>MEQRETIMLPGSDYNHWLIVMEFPKDPAPSRDQMIDTYLNTLATVLGSMEEAKKNMYAFSTTTYTGFQCTIDEETSEKFKGLPGVLWVLPDSYIDVKNKDYGGDKYINGEIIPSTYPTYQPKQLEHHHHHHHH[3x];> HMELFAELRRQGVAPTVVTYNTLIDGLCKAGKLDEALKLFEEMVEKGIKPDEFTFSSVLKACARLGALELGKQIHGYVIKSGFEGNVVVYNALIDMYSKCGLLEEARKVFDEMPEKDVVTYNTLIDGLCKAGKLDEALKLFEEMVEKGIKPDEFTFSSVLKACARLGALELGKQIHGYVIKSGFESNVVVYNALIDMYSKCGLLE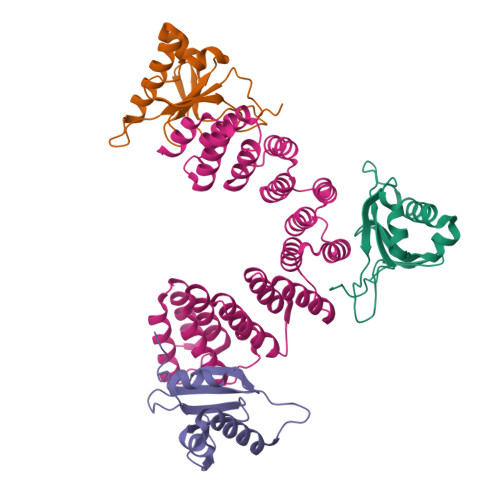EARKVFDEMPEKDVVTYNTLIDGLCKAGKLDEALKLFEEMVEKGIKPDEFTFSSVLKACARLGALELGKQIHGYVIKSGFESNVVVYNALIDMYSKCGLLEEARKVFDEMPEKDELTYRRVVESYCRAKRFELEHHHHHHHH>[2x]ADLGSLVPRGSAMGTNQLDIC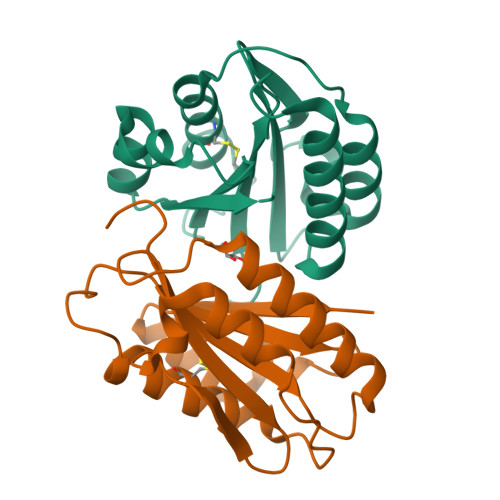FLIDSSGSIGIQNFRLVKQFLHTFLMVLPIGPEEVNNAVVTYSTDVHLQWDLQSPNAVDKQLAAHAVLDMPYKKGSTNTSDGLKACKQILFTGSRPGREHVPKLVIGMTDGESDSDFRTVRAAKEIRELGGIVTVLAVGHYVAAALVPRGSHHHHHH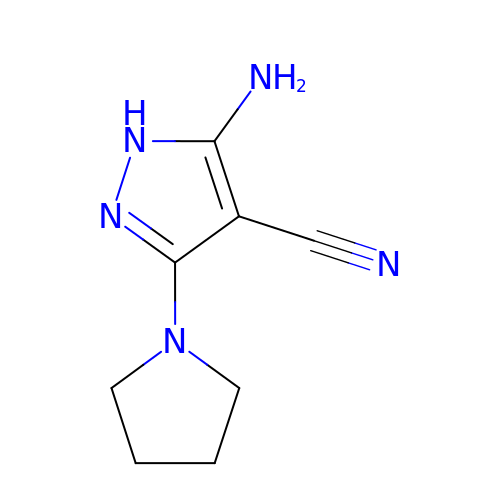5-azanyl-3-pyrrolidin-1-yl-1~{H}-pyrazole-4-carbonitrile | C8 H11 N5 | RQDSNKYYHIZWJX-UHFFFAOYSA-N>MNRIFFILVAAGVPLSVIGSLMHWPSAVLFAVYCVTIIALASYMGRATESLSIIAGPRIGGLLNATFGNAVELIISMFALKEGLTGIVLASLTGSVLGNLLL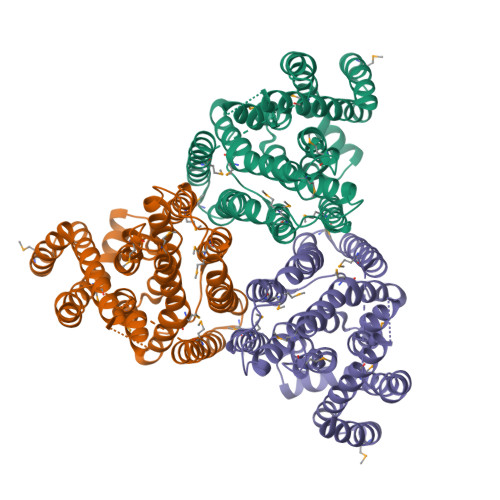VAGLSFFVGGLKYARQEFNIHDARHNSGLLIFAIIVAFVIPEVFSVGMGNASKLNLSIGISIIMILLYVAALYFKLVTHRGVYQPNNAAQTEEEEEPEWSGKVATIVLFAATIVVAYISENLVHTFHSVAEQFGWSELFIGVIIVAIVGNAAEHASAIIMAFKNKMDIAVEIAVGSTLQIAMFVAPVLVICSIFFPTSMPLVFTLPELVAMVSAVLLMIAISNDGDSNWFEGATLLAAYVIMAIGFFLL[2x]>EAETRECIYYNANWELERTNQSGLERCEGEQDKRLHCYASWRNSSGTIELVKKGCWLDDFNCYDRQECVATEENPQVYFCCCEGNFCNERFTHLPEPG[2x];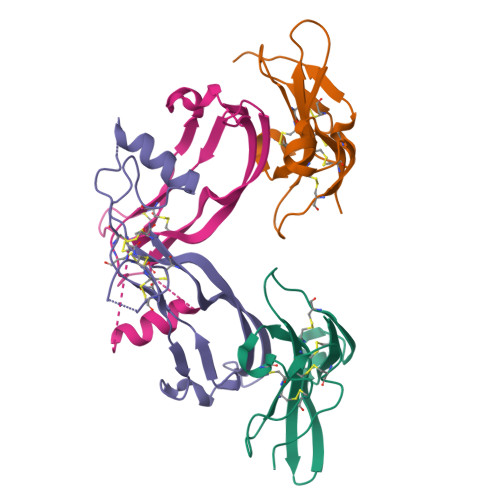>GLECDGKVNICCKKQFFVSFKDIGWNDWIIAPSGYHANYCEGECPSHIAGTSGSSLSFHSTVINHYRMRGHSPFANLKSCCVPTKLRPMSMLYYDDGQNIIKKDIQNMIVEECGCS[2x]>[9x]MAAQATAETPAGELPVIDAVTTHAPEVPPAIDRDYPAKVRVKMETVEKTMKMDDGVEYRYWTFDGDVPGRMIRVREGDTVEVEFSNNPSSTVPHNVDFHAATGQGGGAAATFTAPGRTSTFSFKALQPGLYIYHCAVAPVGMHIANGMYGLILVEPKEGLPKVDKEFYIVQGDFYTKGKKGAQGLQPFDMDKAVAEQPEYVVFNGHVGAIAG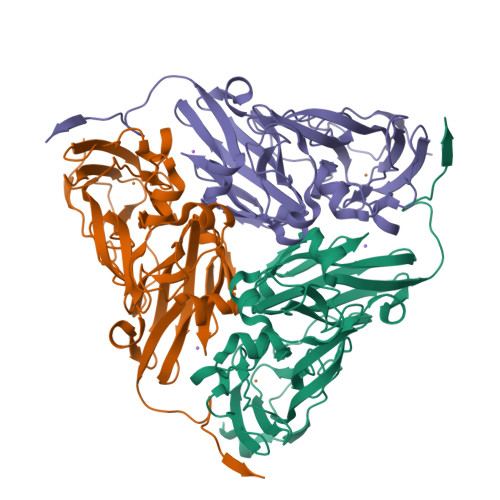DNALKAKAGETVRMYVGNGGPNLVSSFHVIGEIFDKVYVEGGKLINENVQSTIVPAGGSAIVEFKVDIPGNYTLVDHSIFRAFNKGALGQLKVEGAENPEIMTQKLSDTAYAVPRGSLEHHHHHH>[3x]AHHHHHHPGGPGSENLYFQGGSTGGVPIQKVQDDTKTLIKTIVTRINDISHTQSV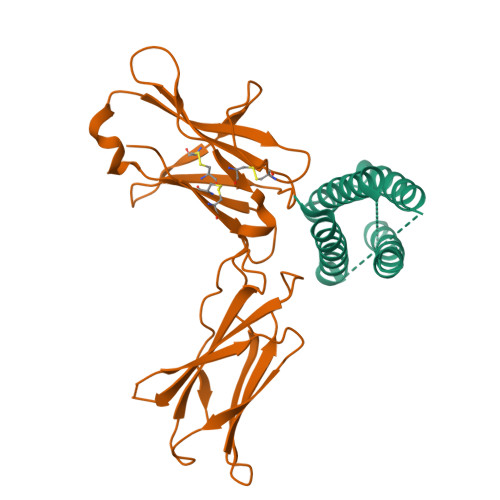SSKQKVTGLDFIPGLHPILTLSKMDQTLAVYQQILTSMPSRNVIQISNDLENLRDLLHVLAFSKSCHLPWASGLETLDSLGGVLEASGYSTEVVALSRLQGSLQDMLWQLDLSPGC;>AHHHHHHPGGPGSENLYFQGGSSGIDVNINISCETDGYLTKMTCRWSTSTIQSLAESTLQLRYHRSSLYCSDIPSIHPISEPKDCYLQSDGFYECIFQPIFLLSGYTMWIRIQHSLGSLDSPPTCVLPDSVVKPLPPSSVKAEITINIGLLKISWEKPVFPENNLQFQIRYGLSGKEVQWKMYEVYDAKSKSVSLPVPDLSAVYAVQVRCKRLDGLGYWSNWSNPAYTVVMD[3x]> GVSDIQEAVAQIKAAGPSKPRLARDPVNQPMINNWVEAIGDRNPIYVDDAAARAAGHPGIVAPPAMIQVWTMMGLGGVRPKDDPLGPIIKLFDDAGYIGVVATNCEQTYHRYLLPGEQVS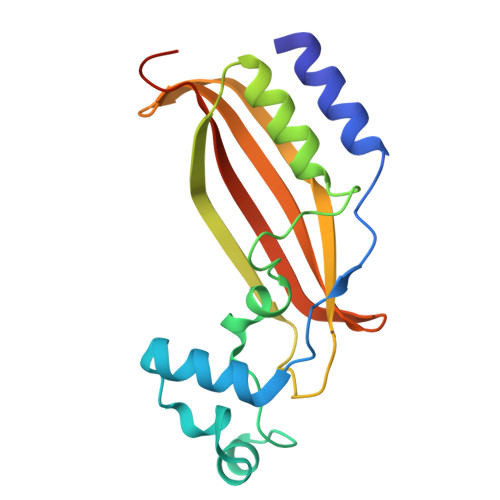ISAELGDVVGPKQTALGEGWFINQHIVWQVGDEDVAEMNWRILKFKPAGSPSSVPDDL> GSHMEFGIDLEFDADVQTMSPEASEYETCYVTSHKGPCRVATYSRDGQLIATGSADASIKILDTERMLAKSAMPIEVMMNETAQQNMENHPVIRTLYDHVDEVTCLAFHPTEQILASG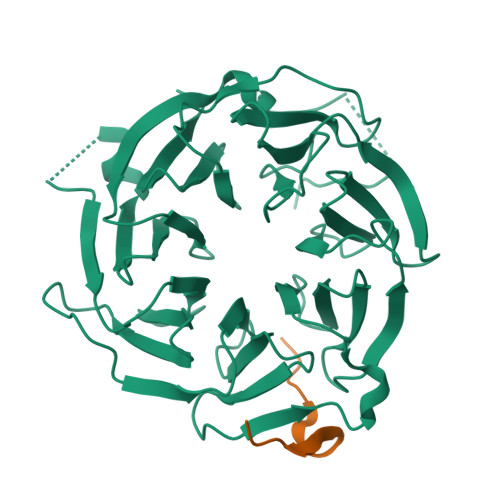SRDYTLKLFDYSKPSAKRAFKYIQEAEMLRSISFHPSGDFILVGTQHPTLRLYDINTFQCFVSCNPQDQHTDAICSVNYNSSANMYVTGSKDGCIKLWDGVSNRCITTFEKAHDGAEVCSAIFSKNSKYILSSGKDSVAKLWEISTGRTLVRYTGAGLSGRQVHRTQAVFNHTEDYVLLPDERTISLCCWDSRTAERRNLLSLGHNNIVRCIVHSPTNPGFMTCSDDFRARFWYRRSTTD;> YPKPDTQQMIPFQPRHLAPP>GDDEEADDPIRMYFEPGHYTVMENCGEFEVRVVRRGDISTYASVEYETQDGTASAGTDFVGRKGLLSFPPGVDEQRFRIEVIDDDVFEEDECFYIRLFNPSEGVKLAVPMIATVMILDDDHAGIFAFTDSVFEITESVGRFELKVMRYSGARGTVIVPYWTENDTATESKDYEGARGELVFENNESEKFIDLFILEESSYEKDVSFKVHIGEPRLAPDSTHYPKIKEVEKKPVQDLTELDRILLLSKPRNGEL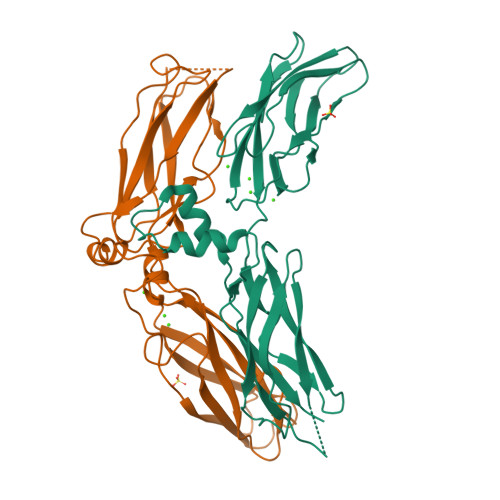TTAYVRIRESQEFKATVDKLVAKANVSAVLGTSSWKEQFKDALTV[4x]>[4x]MGKIKIGINGFGRIGRLVARVALQSEDVELVAVNDPFITTDYMT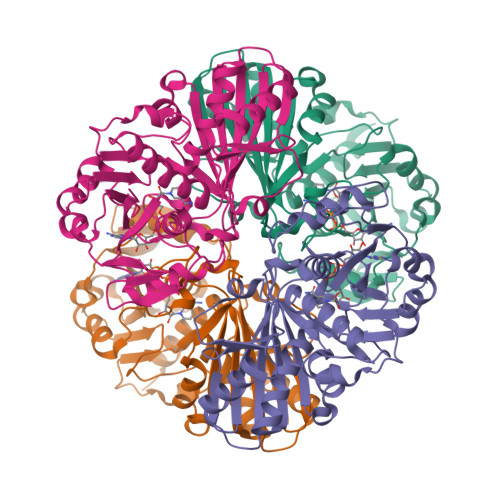YMFKYDTVHGQWKHSDIKIKDSKTLLLGEKPVTVFGIRNPDEIPWAEAGAEYVVESTGVFTDKEKAAAHLKGGAKKVVISAPSKDAPMFVCGVNEDKYTSDIDIVSNASCTTNCLAPLAKVIHDNFGIIEGLMTTVHAITATQKTVDGPSSKDWRGGRAASFNIIPSSTGAAKAVGKVLPDLNGKLTGMSFRVPTVDVSVVDLTVRIEKAASYDAIKSAIKSASEGKLKGIIGYVEEDLVSTDFVGDSRSSIFDAKAGIALNDNFVKLVAWYDNEWGYSNRVIDLIRHMAKTQ> MKKLIPILEKIPEVELPVKEITFKEKLKWTGIVLVLYFIMGCIDVYTAGAQIPAIFGGTLITLGIGPIVTAGIIMQLLVGSGIIQMDLSIPENRALFQGCQKLLSIIMCFVEAVLFVGAGAFGILTPLLAFLVIIQIAFGSIILIYLDEIVSKYGIGSGIGLFIAAGVSQTIFVGALGPEGYLWKFLNSLIQGVPNIEYIAPIIGTIIVFLMVVYAECMRVEIPLAHGRIKGAVGKYPIKFVYVSNIPVILAAALFANIQLWGLALYRMGIPILGHYEGGRAVDGIAYYLSTPYGLSSVISDPIHAIVYMIAMIITCVMFGIFWVETTGLDPKSMAKRIGSLGMAIKGFRKSEKAIEHRLKRYIPPLTVMSSAFVGFLATIANFIGALGGGTGVLLTVSIVYRMYEQLLREKVSELHPAIAKLLNK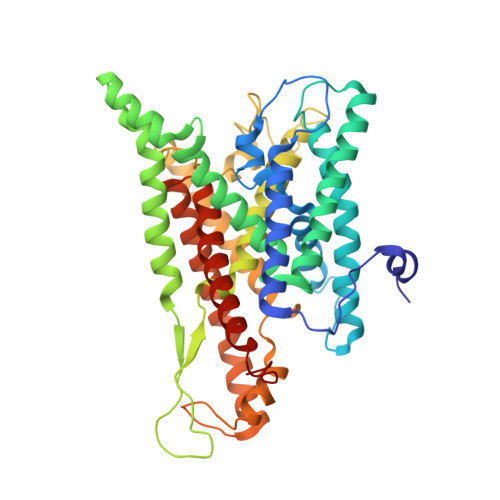;> MKTDFNQKIEQLKEFIEECRRVWLVLKKPTKDEYLAVAKVTALGISLLGIIGYIIHVPATYIKGILKPPTTPRV;> MSKREETGLATSAGLIRYMDETFSKIRVKPEHVIGVTVAFVIIEAILTYGRFL>MLGRIWLPVLIVVAVAAGALIVMNVRTVFGSNPVVVTEKTSDNAEDFNPKVVTYEIFGSGSSAVINYMDLEGMPQRVESTPLPWSLTLQTTLPSVMPHIMAQGDGDSITCRVTVDDVVKEERTATGMNAETFCYVKAA[3x];>[3x]MSAPTDDTPTDAIAAPRHSAPPRPRLPWFLRTFAVPIILAWVAVVAILNTVVPTLDEVGEMRAVSMAPNDAPSTLAIKRVGQVFEEYDTSSSVMIVLEGEEPLGIEAHAFYDKMVADLRADTEHVQHVQDFWGDTLTASGAQSVDGKAAYVQVYIAGDQGESLANESVEAVRKIATERETPSGVKAYVTGAAATSADQRAEGDASMKLIEGVTFAVITVMLLAVYRSVITTLIVLAMVVLGLSGARGIVAFLGFYNVFGLTTFATNMVVTLAIAAATDYAIFLIGRYQEARRAGEDRESAYYTMFHGTAHVVLASGLTIAGATLCLHFTRLPYFQTMGVPLAIGMLIVVAAALTAGPAVISVVSRFGKTLEPKRFSRSPGWHRVGTATVRWPGAILVCAVVAALIGLLALPGYYTTYDDRRYLPDDVPANVGYDAAFRHFSQAKMNPDLMMVETDRDLRNPADFLVIDKIAKALKNVHGIAQVQTITRPDGDPIEHSTIPYTIGQSGTTQIMNNDYMQTNLDNLLKQADDLQTSIDSMTEMMNIQTELAAVSQSMADKMAQTSDDTADVRDHLADFDDFFRPIRNYLYWEPHCYDIPMCWSMRSIFESIDGINTMSDDFQELVPEMRRMADLMPRMVAVMPAQIQSMKNQKQTLLNQYQVQKAQQDQNMAMQENATAMSQAFDAAKNDDSFYLPPEAFETDDFQRGMKLFMSPDGHAVRFTIIHQGDPLTEEGTARMDELKVAAADAIKGTPFEGARIYLGGSAATYNDMQIGADYDLIIVAASALILIFIIMMVLTRAVVAAAVIVGTVVLSLASAFGLSVLLWQHIVGIPLHWMVLPMSVIVLLAVGADYNLLLVSRMKEEIHAGIRTGIIRAMVGTGAVVTAAGLVFAFTMASMAVSSLITIGQVGTTIGLGLLFDTLVVRSLMTPSIATLLGRWFWWPQRVRERPVPSKWPTPIQRTPEEALS;>[3x]MAATQEEIIAGLAEIIEEVTGIEPSEVTPEKSFVDDLDIDSLSMVEIAVQTEDKYGVKIPDEDLAGLRTVGDVVAYIQKLEEENPEAA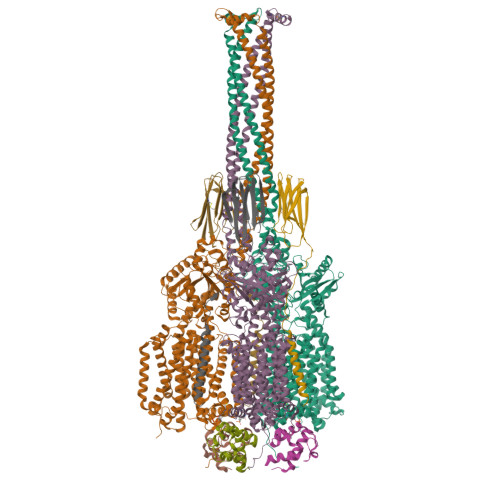AALREKFAADQ>[2x]KPVSLSYRCPCRFFESHVARANVKHLKILNTPNCALQIVARLKNNNRQVCIDPKLKW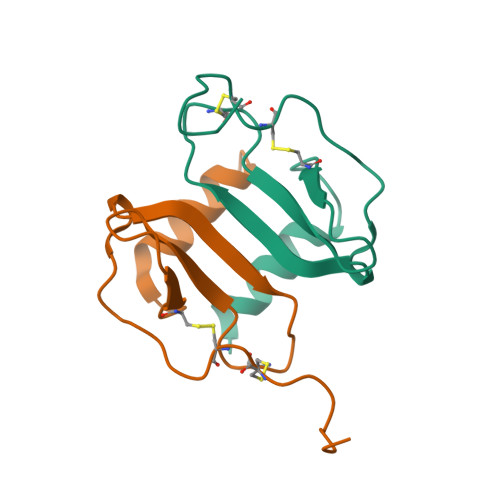IQEYLEKALNK>MVNNNRPRRQRAQRVVVTTTQTAPVPQQNVPRNGRRRRNRTRRNRRRVRGMNMAALTRLSQPGLAFLKCAFAPPDFNTDPGKGIPDRFEGKVVSRKDVLNQSISFTAGQDTFILIAPTPGVAYWSASVPAGTFPTSATTFNPVNYPGFTSMFGTTSTSRSDQVSSFRYASMNVGIYPTSNLMQFAGSITVWKCPVKLSTVQFPVATDPATSSLVHTLVGLDGVLAVGPDNFSESFIKGVFSQSACNEPDFEFNDILEGIQTLPPANV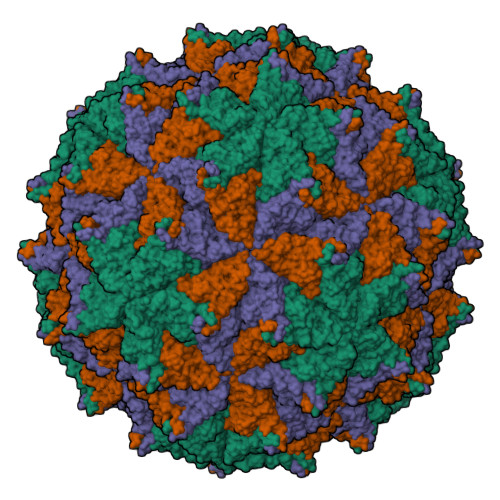SLGSTGQPFTMDSGAEATSGVVGWGNMDTIVIRVSAPEGAVNSAILKAWSCIEYRPNPNAMLYQFGHDSPPLDEVALQEYRTVARSLPVAVIAAQTASMWERVKSIIKSSLAAASNIPGPIGVAASGISGLSALFEGFGF[3x]> APVKYGELIVLGYNGSLPNGDRGRRKSRFALFKRPKANGVKPSTVHIACTPQAAKAISNKDQHSISYTLSRAQTVVVEYTHDSNTDMFQIGRSTESPIDFVVTDTVPGSQSNSDTQSVQSTISRFACRIICERNPPFTARIYAAGFDSSKNIF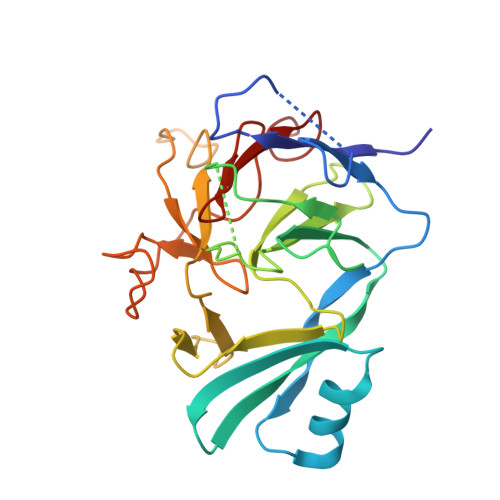LGEKAAKWKTSDGQMDGLTTNGVLVMHPRNGFTEDSKPGIWREISVCGNVFSLRETRSAQQRGKMVEIETNQLQDGSLIDLCGATLLWRTAEGLSHTP> MAGTDKRKQSLYFPEEMLKEIQEEATRQDRSLSWVVQQAWKIARERIKSFPAVNDVTGDERQDPREE

We show that CdbA is a tetrameric ribbon-helix-helix DNA binding protein and changes conformation upon c-di-GMP binding. Consistently, c-di-GMP and DNA binding are mutually exclusive. In vivo CdbA is essential, while CdbB is not, and depletion of CdbA causes defects in chromosome organization and segregation resulting in defects in cell division. CdbA is abundant and binds globally to the M. xanthus chromosome. These observations are in agreement with a model whereby CdbA is a ligand-regulated nucleoid-associated protein (NAP) important for chromosome organization and segregation and in which CdbA activity is modulated by c-di-GMP.

We obtained two crystal forms of full-length CdbA-His6. The first structure (traced residues 5–52) verified that CdbA is a RHH superfamily member, with crystallographic symmetry generating a classical RHH dimer. In CdbA, the exposed face of the β-strand projects residues K8, S10 and Y12, while L11 and F13 are facing the hydrophobic core of the dimer. The β-strand is terminated by P14, leading into α-helix1 (residues 16-28), followed by a loop and then α-helix2 (residues 32–48), with a strongly kinked region at A43/R44, and a C-terminal tail traceable to A52. The two α2 helices run antiparallel, with kink residues I42 and A43 packing against their counterparts in the opposing chain. Successful model building of the first form allowed us to solve the second form via molecular replacement. Upon solving this crystal form, we realized that a similar, but more loosely-packed, tetramer can be observed when considering the crystal symmetry of form one. The tetramer interface displays different hydrophobic packing between the two crystal forms we observed here, suggesting that it may have inherent plasticity that allows it to undergo this change.(4aR,7aR)-6-(pyrimidin-2-yl)-7a-(thiophen-2-yl)-4,4a,5,6,7,7a-hexahydropyrrolo[3,4-d][1,3]thiazin-2-amine 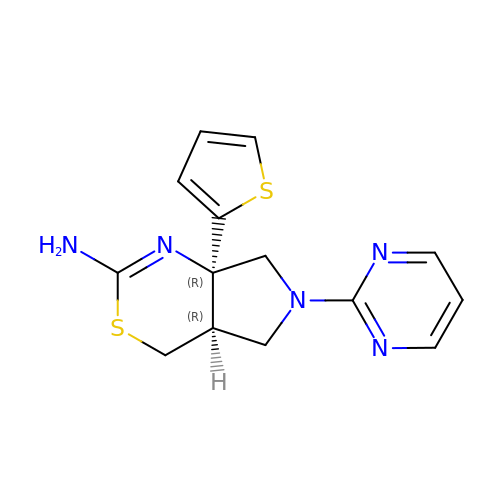| C14 H15 N5 S2 | GFWNXZDRVLVYFN-HZMBPMFUSA-N>MKNTTTYDYIVVGGGTSGLVVANRLSENPDVSVLLLEAGASVFNNPDVTNANGYGLAFGSAIDWQYQSINQSYAGGKQQVLRAGKALGGTSTINGMAYTRAEDVQIDVWQKLGNEGWTWKDLLPYYLKSENLTAPTSSQVAAGAAYNPAVNGKEGPLKVGWSGSLASGNLSVALNRTFQAAGV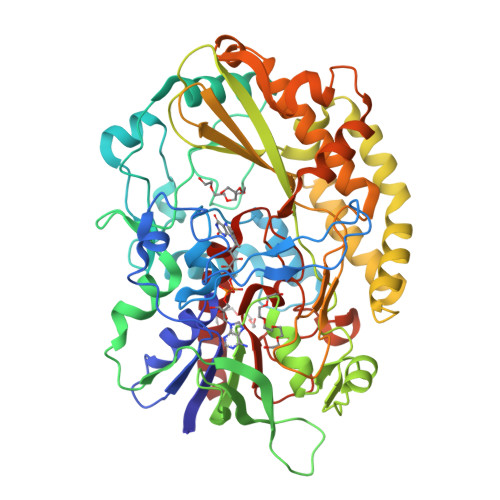PWVEDVNGGKMRGFNIYPSTLDVDLNVREDAARAYYFPYDDRKNLHLLENTTANRLFWKNGSAEEAIADGVEITSADGKVTRVHAKKEVIISAGALRSPLILELSGVGNPTILKKNNITPRVDLPTVGENLQDQFNNGMAGEGYGVLAGASTVTYPSISDVFGNETDSIVASLRSQLSDYAAATVKVSNGHMKQEDLERLYQLQFDLIVKDKVPIAEILFHPGGGNAVSSEFWGLLPFARGNIHISSNDPTAPAAINPNYFMFEWDGKSQAGIAKYIRKILRSAPLNKLIAKETKPGLSEIPATAADEKWVEWLKANYRSNFHPVGTAAMMPRSIGGVVDNRLRVYGTSNVRVVDASVLPFQVCGHLVSTLYAVAERASDLIKEDAKSA[2x]>[4x]MARPKSEDKKQALLEAATQAIAQSGIAASTAVIARNAGVAEGTLFRYFATKDEL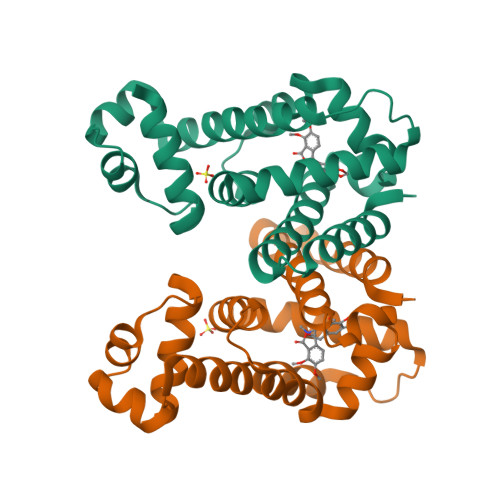INTLYLHLTHDMCQSLIMELDRSITDAKMMTRFIWNSYISWGLNHPARHRAIRQLAVSEKLTKETRQRARDMFPELRDLCYRSLLMVFMSDEYRAFGDGLFMALAETTMDFAARDPARAGEYIALGFEAMWRALTREEQ>NLKVEFYNSNPSDTTNSINP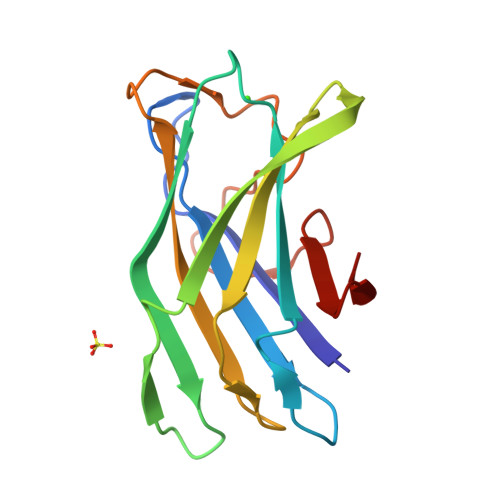QFKVTNTGSSAIDLSKLTLRYYYTVDGQKDQTFWCDHAAIIGSNGSYNGITSNVKGTFVKMSSSTNNADTYLEISFTGGTLEPGAHVQIQGRFAKNDWSNYTQSNDYSFKSASQFVEWDQVTAYLNGVLVWG[2x]> GAMGESLSIYKSGLKNDFQDWSWGEHSLTDTTNVESGETNSISFTPKAYGAVFLGCFECIDTD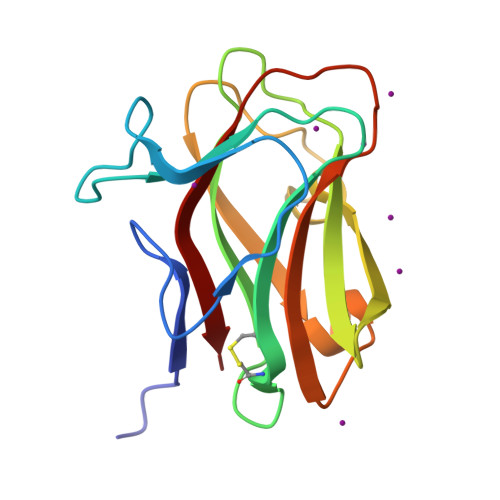TYNNIEFDINGGSSGAQLLRITVVKNSKSVGSKLITDLNGGTPIEANSWTKIKASFIDDFKVSGKVDGIWIQDIKGDTQSTVYISNIIATA>[32x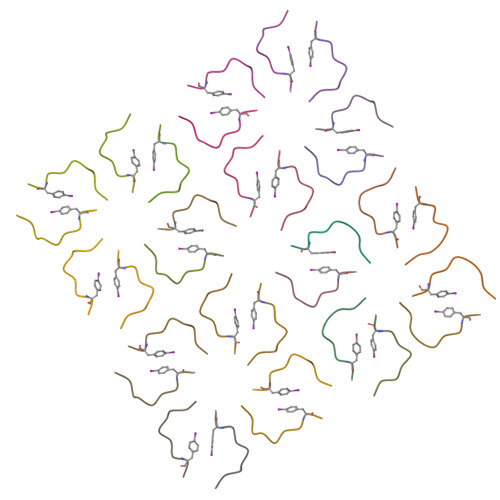]GFGGNDNFG> SNQRMNDYSQPESQSDLAPKSSTIQPQPQPLLSKTPSMSLNLLSSSGPNRQVLPSEPSNFMTLMGQNGALLTVWALAKRNWLWAYPNIYSQDFGNIRNWKMEPGKHREYFRFVNQSLGTCVEAYGNGLIHDICSLDKLAQEFELLPTDSGAVVIKSVSQGRCVTYNPVSTTFYSTVTLSVCDGATEPSRDQTWYLAPPVLEATAVN;> NLSDFKVATWNLQGSSAVNESKWNINVRQLLSGEQGADILMVQEAGSLPSSAVRTSRVIQHGGTPIEEYTWNLGTRSRPNMVYIYYSRLDVGANRVNLAIVSRRQADEAFIVHSDSSVLQSRPAVGIRIGTDVFFTVHALATGGSDAVSLIRNIFTTFNSSSSPPERRVYSWMVVGDFNRAPANLEVALRQEPAVSENT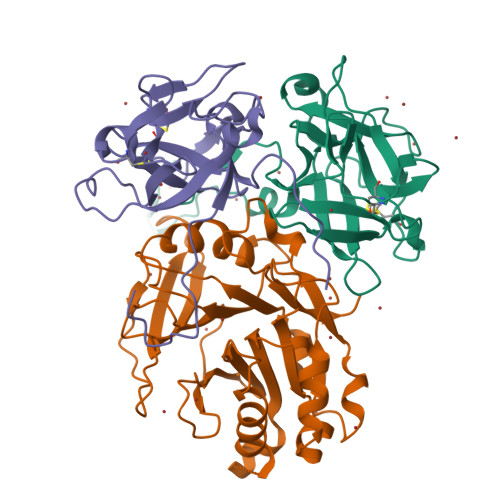IIIAPTEPTHRSGNILDYAILHDAHLPRREQARERIGASLMLNQLRSQITSDHFPVSFVRDR;> ESNPDPTTYPDVELSPPPRISLRSLLTAQPVKNDHYDSHNYLSTHWELIDYKGKEYEKLRDGGTLVQFKVVGAAKCFAFLGKGTTDCKDTDHTVFNLIPTNTGAFLIKDALLGFCITSHDFDDLKLEPCGGSVSGRTFSLAYQWGILPPFGPSKILIPPVRRNQGS>MASDHQTQAGKPQSLNPKIIIFEQENFQGHSHELNGPCPNLKETGVEKAGSVLVQAGPWVGYEQANCKGEQFVFEKGEYPRWDSWTSSRRTDSLSSLRPIKVDSQEHKIILYENPNFTGKKMEIIDDDVPSFHAHGYQEKVSSVRVQSGTWVGYQYPGYRGLQYLLEKGDYKDSSDFGA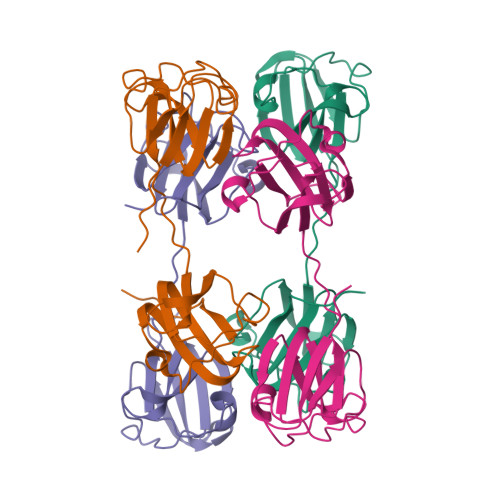PHPQVQSVRRIRDMQWHQRGAFHPSN[12x]> AMADITSLYKKAGSAAAPFTYWLNPEIYDAGGLSRRAFPEGFVFGTAASAYQVEGMAKQGGRGPSIWDAFIEKPGTIPNNATADVTVDEYHRYKEDVNIMKNMGFDAYRFSISWSRIFPNGTGMVNQEGVDYYNRLIDYMVKKGIKPYANLYHYDLPLALHEQYLGWLSPNIVEAFADYAD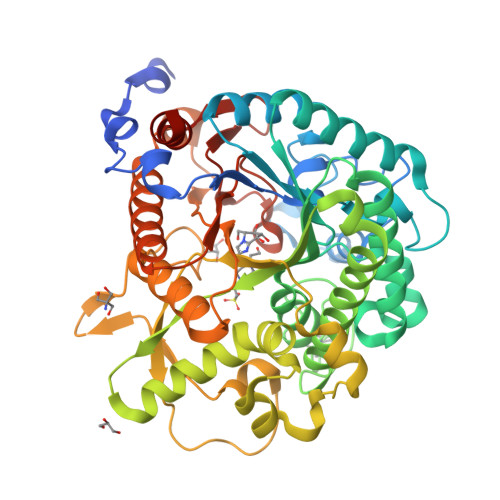FCFQTFGDRVKDWFTFNEPRCVAALGYDNGFHAPGRCSGCDAGGNSTTEPYLAAHHLILSHAAAVKRYREKYQLYQKGRIGILLDFVWYEPFSDSNADRAAAQRARDFHLGWFLDPIIHGRYPYSMLEIVKDRMPTFSDEESRMVKDSIDYVGINHYTSFYMKDPGPWNLTPTSYQDDWHVGFAYERNGVPIGAQANSYWLYIVPWGINKAVTYVKETYGNPTMILSENGMDQPGNVSITQGVHDTVRIRYYRNYITELKKAIDDGAKVIGYFAWSLLDNFEWRLGYTSRFGIVYVDYKTLKRYPKDSAFWFKNMLSSKKRN> SRAPYSGPQDLAALLEQIGCLKYLQVFE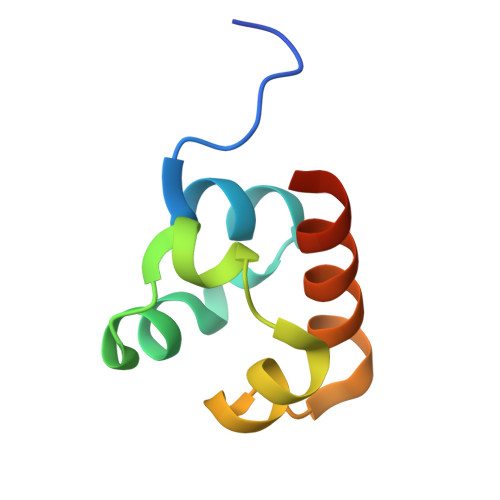EQDVDLREFLTLTESDLKEIGITLFGPKRKMTSAIARWHSSAR> MSSIIRKIINTSKAPAAIGPYSQAVVVDRTMYVSGQLGMDPA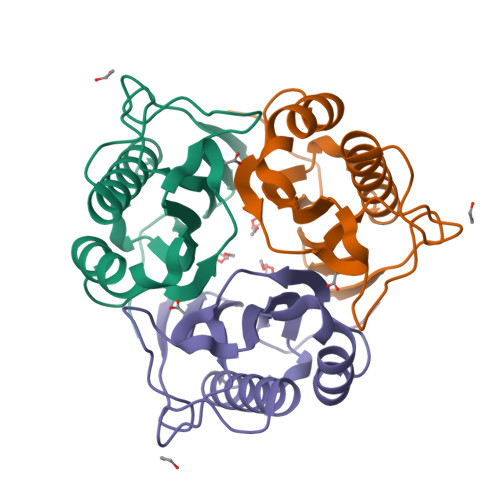SGQLVEGGVQAQTKQALVNMGEILKEAGCGYDSVVKTTVLLADMNDFASVNDVYKTFFSSSFPARAAYQVAALPRGGLVEIEAVAVLGPLTEVS> MPRVKLGTQGLEVSKLGFGCMGLSGDYNDALPEEQGIAVIKEAFNCGITFFDTSDIYGENGSNEELLGKALKQLPREKIQVGTKFGIHEIGFSGVKAKGTPDYVRSCCEASLKRLDVDYIDLFYIHRIDTTVPIEITMGELKKLVEEGKIKYVGLSEASPDTIRRAHAVHPVTALQIEYSLWTRDIEDEIVPLCRQLGIGIVPYSPIGRGLFWGKAIKESLPEN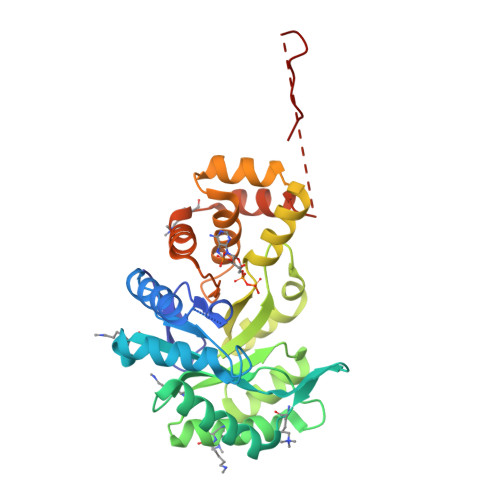SVLTSHPRFVGENLEKNKQIYYRIEALSQKHGCTPVQLALAWVLHQGEDVVPIPGTTKIKNLHNNVGALKVKLTKEDLKEISDAVPLDEVAGESIHEVIAVTNWKFANTPPLK>MAKGKSEVVEQNHTLILGWSDKLGSLLNQLAIANESLGGGTIAVMAERDKEDMELDIGKMEFDFKGTSVICRSGSPLILADLKKVSVSKARTIIVLAEDGNADQSDARALRTVLSLTGVKEGLRGHIVVE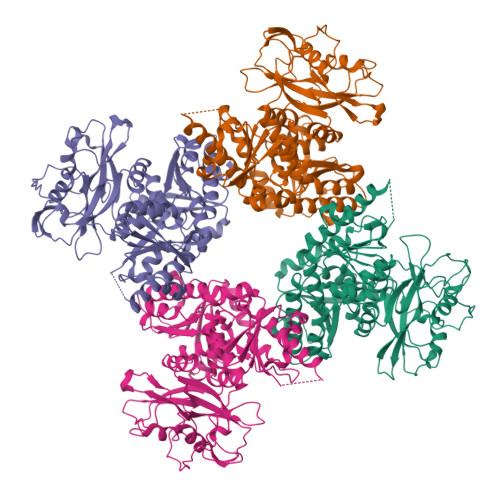MSDLDNEVLVKLVGGDLVETVVAHDVIGRLMIQCARQPGLAQIWEDILGFENCEFYIKRWPQLDGMLFEDVLISFPAAIPCGIKVASYGGKIILNPDDSYVLQEGDEVLVIAEDDDTYAPAPLPMVRRGSLPKDFVYPKSPERILFCGWRRDMEDMITVLDASLAPDSELWMFNDVPEKEREKKLIDGGLDISRLENISLVNREGNAVIRRHLESLPLESFDSILILADESVEDSAIQADSRSLATLLLIRDIQARRLPYVAMASQTQGGNFSKGSWIGEMKQASDKTVIISEILDPRTKNLLSMSKISDYVLSNELVSMALAMVAEDRQINDVLEELFAEEGNEMHIRQADIYLREGEEMSFYEIMLRARQRREILIGYRLANAERAVINPPAKTGRRKWSLKDVFVVITEKEGSRSHHHHHH[4x]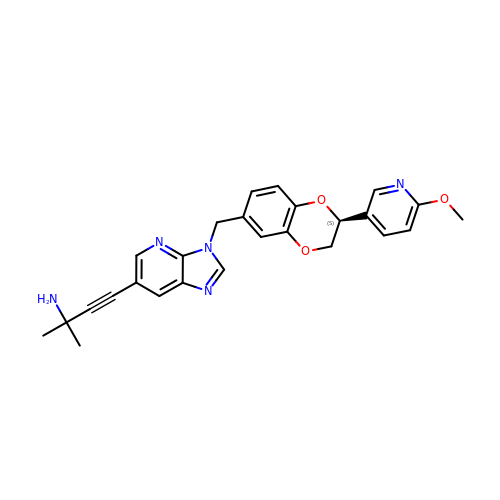4-(3-{[(2S)-2-(6-methoxypyridin-3-yl)-2,3-dihydro-1,4-benzodioxin-6-yl]methyl}-3H-imidazo[4,5-b]pyridin-6-yl)-2-methylbut-3-yn-2-amine | C26 H25 N5 O3 | DRBFONOVLOXKJM-HSZRJFAPSA-N>[2x]MDLKIKNKVCIITGGAKGIGYGIAKLWASEGGIPVIFSRSMPKEHDKELKKLSSEYEFYEIDLKNYEQIEKLVKKVAIKHGGIYALVNNAGTNDNLHIENTSTQDLIKSYENNLFHYYTMTKECLPYIKKEQGSILNIVSKTGITGQGRTSAYASAKAAQMGFTREWACAFAKDNVRVNAIAPAEVM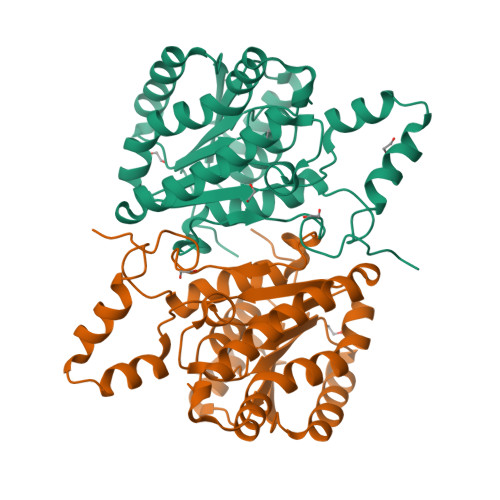TPLYEKWLQNFPNPKEQYEKIAKAIPLGHRFTTIEEIANTAVFTLSPLASHTTGQILMPDGGYVHLDRALNWDENTRGHHHHHH>[4x]AYTFDSTMLDTNSGESIDVSLFNQGLQLPGNYFVNVFVNGRKVDSGNIDFRLEKHNGKELLWPCLSSLQLTKYGIDIDKYPDLIKSGTEQ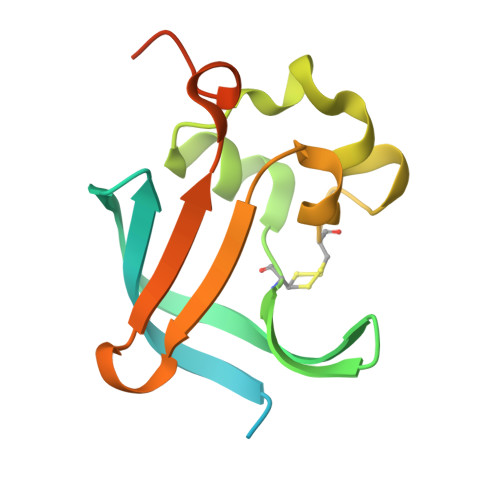CVDLLAIPHSDVQFYFNQQKLSLIVPPQALLPRFDGIMPMQLWDDG>GMSRAPDTWILTADCPSMLGTVDVVTRYLFEQRCYVTEHHSFDDRQSGRFFIRVEFRQPDDFDEAGFRAGLAERSEAFGMAFELTAPNHRPKVVIMVSKADHCLNDLLYRQRIGQLGMDVVAVVSNHPDLEPLAHWHKIPYYHFALDPKDKPGQERKVLQVIEETGAELVILARYMQVLSPELCRRLDGWAINIHHSLLPGFKGAKPYHQAYNKGVKMVGATAHYIN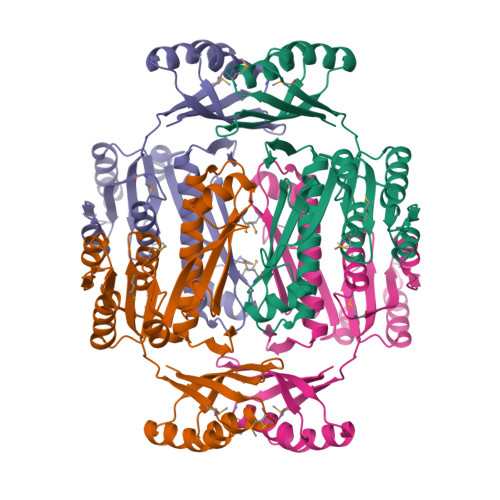NDLDEGPIIAQGVEVVDHSHYPEDLIAKGRDIECLTLARAVGYHIERRVFLNANRTVVL[4x]> EVKLILYHWTHSFSSQKVRLVIAEKALKCEEHDVSLPLSEHNEPWFMRLNSTGEVPVLIHGENIICEATQIIDYLEQTFLDERTPRLMPDKESMYYPWVQHYRELLDSLPMDAYTHGCILHPELTVDSMIPAYATTRIRSQIGNTESELKKLAEENPDLQEAYIAKQKRLKSKLLDHDNVKYLKKILDELEKVLDQVETELQRRNEETPEEGQQPWLCGESFTLADVSLAVTLHRLKFLGFARRNWGNGKRPNLETYYERVLKRKTFNKVLGHVNNILIS

Charcot–Marie–Tooth disease (CMT) is the most common inherited peripheral polyneuropathy in humans, and its different subtypes are linked to mutations in dozens of different genes. Mutations in ganglioside‐induced differentiation‐associated protein 1 (GDAP1) cause two types of CMT, demyelinating CMT4A and axonal CMT2K. The GDAP1‐linked CMT genotypes are mainly missense point mutations. Structural analysis of GDAP1 indicates that CMT may arise from disruption of specific intra‐ and intermolecular interaction networks, leading to alterations in GDAP1 structure and stability, and, eventually, insufficient motor and sensory neuron function.

Here, we describe the biochemical and structural properties of the Finnish founding CMT2K mutation H123R and CMT2K‐linked R120W, both of which are autosomal dominant mutations. The disease variant proteins retain close to normal structure and solution behavior, but both present a significant decrease in thermal stability. Using GDAP1 variant crystal structures, we identify a side‐chain interaction network between helices ⍺3, ⍺6, and ⍺7, which is affected by CMT mutations, as well as a hinge in the long helix ⍺6, which is linked to structural flexibility.>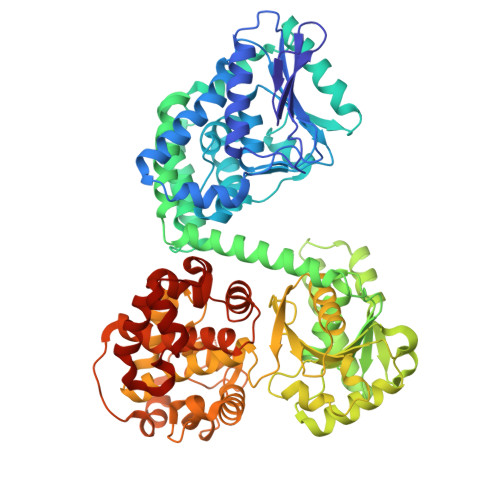 MIYEGKAITVTALESGIVELKFDLKGESVNKFNRLTLNELRQAVDAIKADASVKGVIVSSGKDVFIVGADITEFVENFKLPDAELIAGNLEANKIFSDFEDLNVPTVAAINGIALGGGLEMCLAADFRVMADSAKIGLPEVKLGIYPGFGGTVRLPRLIGVDNAVEWIASGKENRAEDALKVSAVDAVVTADKLGAAALDLIKRAISGELDYKAKRQPKLEKLKLNAIEQMMAFETAKGFVAGQAGPNYPAPVEAIKTIQKAANFGRDKALEVEAAGFAKLAKTSASNCLIGLFLNDQELKKKAKVYDKIAKDVKQAAVLGAGIMGGGIAYQSASKGTPILMKDINEHGIEQGLAEAAKLLVGRVDKGRMTPAKMAEVLNGIRPTLSYGDFGNVDLVVEAVVENPKVKQAVLAEVENHVREDAILASNTSTISISLLAKALKRPENFVGMHFFNPVHMMPLVEVIRGEKSSDLAVATTVAYAKKMGKNPIVVNDCPGFLVNRVLFPYFGGFAKLVSAGVDFVRIDKVMEKFGWPMGPAYLMDVVGIDTGHHGRDVMAEGFPDRMKDDRRSAIDALYEAKRLGQKNGKGFYAYEADKKGKQKKLVDSSVLEVLKPIVYEQRDVTDEDIINWMMIPLCLETVRCLEDGIVETAAEADMGLVYGIGFPLFRGGALRYIDSIGVAEFVALADQYAELGALYHPTAKLREMAKNGQSFFG>[2x]FDFAVIKELKTAASQYGATAPYTLAIVESVADNWLTPTDWN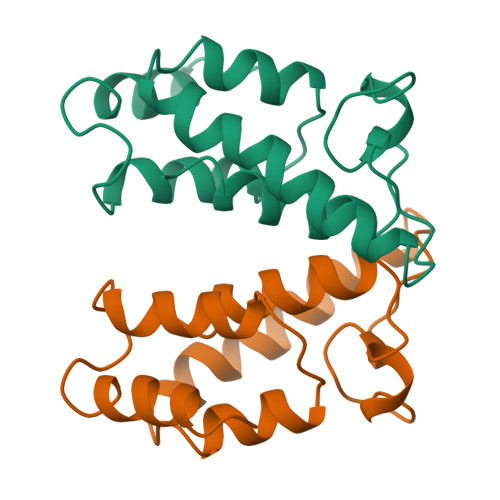TLVRAVLSGGDHLLWKSEFFENCRDTAKRNQQAGNGWDFDMLTGSGNYSSTDAQMQYDPGLFAQIQAAATKAWRK>[4x]SFVEMVDNLRGKSGQGYYVEMTVGSPPQTLNILVDTGSSNFAVGAAPHPFL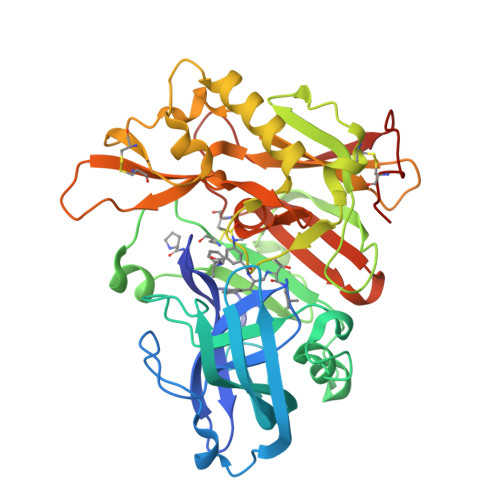HRYYQRQLSSTYRDLRKGVYVPYTQGKWEGELGTDLVSIPHGPNVTVRANIAAITESDKFFINGSNWEGILGLAYAEIARPDDSLEPFFDSLVKQTHVPNLFSLQLCGAGFPLNQSEVLASVGGSMIIGGIDHSLYTGSLWYTPIRREWYYEVIIVRVEINGQDLKMDCKEYNYDKSIVDSGTTNLRLPKKVFEAAVKSIKAASSTEKFPDGFWLGEQLVCWQAGTTPWNIFPVISLYLMGEVTNQSFRITILPQQYLRPVEDVATSQDDCYKFAISQSSTGTVMGAVIMEGFYVVFDRARKRIGFAVSACHVHDEFRTAAVEGPFVTLDMEDCGYN(5P)-5-[2,3-dichloro-4-(1,1,1,3,3,3-hexafluoro-2-hydroxypropan-2-yl)phenyl]-N-(2-hydroxy-2-methylpropyl)-4-[(2S)-2-methylpyrrolidine-1-carbonyl]-1,3-thiazole-2-carboxamide 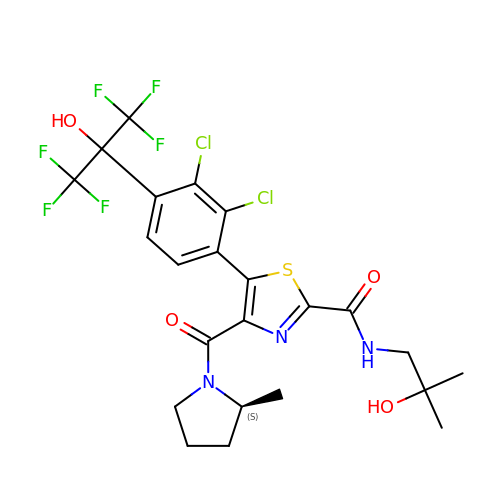| C23 H23 Cl2 F6 N3 O4 S | ZQHVEGQHOKDZEN-JTQLQIEISA-N>SDVFHLGLTKNDLQGATLAIVPGGPDRVEKIAALMDKPVKLASHREFTTWRAELDGKPVIVCSTGIGGPSTSIAVEELAQLGIRTFLRIGTTGAIQPHINVGDVLVTTASVRLDGASLHFAPLEFPAVADFECTTALVEAAKSIGATTHVGVTASSDTFYPGQERYDTYSGRVVRHFKGSMEEWQAMGVMNYEMESATLLTMCASQGLRAGMVAGVIVNR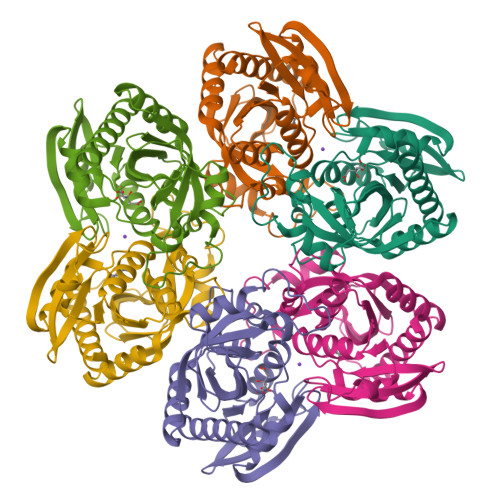TQQEIPNAETMKQTESHAVKIVVEAARRLL[2x]>SNAMDQTIHHQIQQALHFRTAVRVYKEEKISDEDLALILDAAWLSPSSIGLEGWRFVVLDNKPIKEEIKPFAWGAQYQLETASHFILLIAEKHARYDSPAIKNSLLRRGIKEGDGLNSRLKLYESFQKEDMDMADNPRALFDWTAKQTYIALGNMMMTAALLGIDTCPIEGFHYDKVNHILAKHNVIDLEKEGIASMLSLGYRLRDPKHAQVRKPKEEVMSV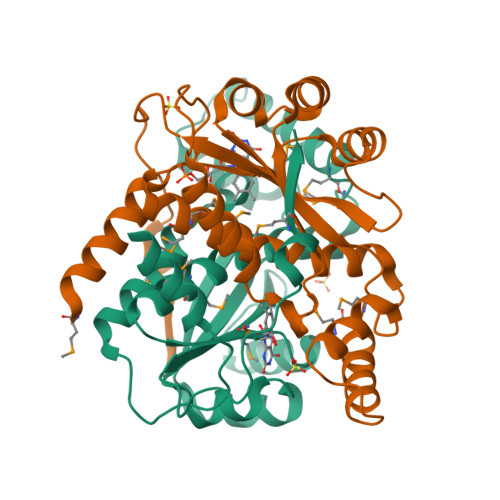VK[4x]> AATSRPERVWPDGVIPFVIGGNFTGSQRAVFRQAMRHWEKHTCVT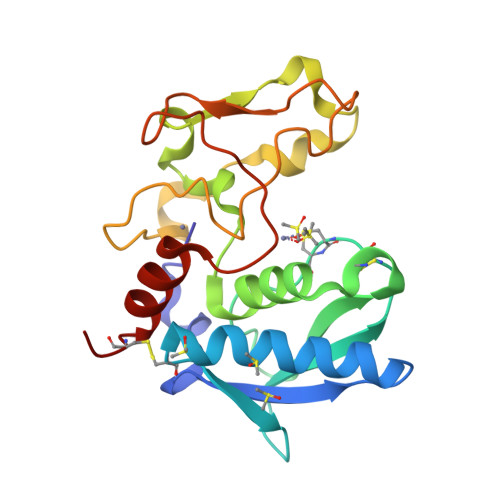FLERTDEDSYIVFTYRPCGCCSYVGRRGGGPQAISIGKNCDKFGIVVHELGHVVGFWHEHTRPDRDRHVSIVRENIQPGQEYNFLKMEPQEVESLGETYDFDSIMHYARNTFSRGIFLDTIVPKYEVNGVKPPIGQRTRLSKGDIAQARKLYKCPA> MACEWLGRYRMISNESLSLLKEMGGKYPEGTKVSFPGRLYNMIDNAKVEDQVKFLVLTLDHIIRLMDAREHMNSVQWNLQTVEHFLTVLNRQSSDLKECVARYQPSHKESYEKKINRHFKILKKNLKKKEYSAQAWEQIRRAVKHHLQRMDIIASIANR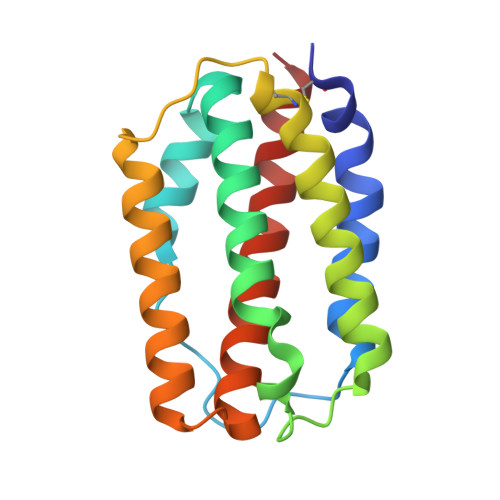R Nipah virus (NiV) and Hendra virus (HeV) are highly pathogenic henipaviruses within the Paramyxoviridae family, causing severe respiratory and neurological diseases in humans and animals with fatality rates up to 75%, and no licensed human vaccines or therapeutics. The majority of candidate vaccines use the attachment glycoprotein G as an antigen, which recognizes the receptors Ephrin B2 or Ephrin B3 on the host cell. The G proteins of NiV (NiV-G) and HeV (HeV-G) have ~80% amino acid homology, which to some extent limits their ability to induce cross-immune antibody responses. HeV-G and NiV-G share a similar beta-propeller structure composed of six “blades”.

Leveraging structure-guided design, we introduced a single amino acid substitution (S586N) in HeV-G to reconstruct this NiV-specific epitope on HeV-G, which generated the HeV-GS586N mutant. Utilizing X-ray crystallography techniques, we successfully generated high-quality protein crystals and determined the crystal structure of the HeV-GS586N. At position 586 of blade6, the nonconserved amino acid S586N was the closest to the 14F8 interacting surface. Compared with wild-type HeV-G, the single amino acid substitution caused the top of blade6 to shift toward the center of the receptor-binding surface by a maximum distance of 9 Å. The substitution modified the local molecular framework to elicit relative shifts in the adjacent amino acids Asp585, Thr583, and Gly584 and changes in the solvent-accessible surface area. Therefore, even though only a single amino acid substitution was introduced, the protein conformation was significantly altered, which can explain the strikingly different antigenicity of the wild-type and mutant proteins. Although Asn586 was not directly involved in the interaction with the 14F8 antibody, shaping the molecular framework contributed to the formation of an immunodominant neutralizing epitope. SDS‒PAGE and SEC demonstrated the homogeneity and purity of HeV-GS586N, HeV-GS586N existed predominantly as a tetramer with a minor dimer population, whereas wild-type HeV-G comprised a mixture of tetramer, dimer, and monomer states. Functional assays and immunogenicity studies in mice and non-human primates demonstrated that HeV-GS586N elicited broad neutralizing responses against both HeV and NiV.

>[2x]ICLQKTTSTILKPRLISYTLPINTREGVCITDPLLAVDNGFFAYSHLEKIGSCTRGIAKQRIIGVGEVLDRGDKVPSMFMTNVWTPPNPSTIHHCSSTYHEDFYYTLCAVSHVGDPILNSTSWTESLSLIRLAVRPKSDSGDYNQKYIAITKVERGKYDKVMPYGPSGIKQGDTLYFPAVGFLPRTEFQYNDSNCPIIHCKYSKAENCRLSMGVNSKSHYILRSGLLKYNLSLGGDIILQFIEIADNRLTIGSPSKIYNSLGQPVFYQASYSWDTMIKLGDVDTVDPLRVQWRNNSVISRPGQSQCPRFNVCPEVCWEGTYNDAFLIDRLNWVSAGVYLNSNQTAENPVFAVFKDNEILYQVPLAEDDTNAQKTITDCFLLENVIWCISLVEIYDTGDNVIRPKLFAVKIPAQCSE(6S)-4-(3-fluoropyridin-2-yl)-6-methylpiperazin-2-one | C10 H12 F N3 O | 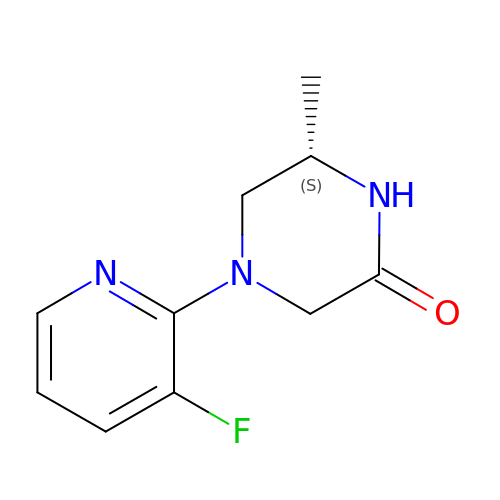ADIKUTCTGUZIDP-ZETCQYMHSA-N>[6x]GPAMASEVLQKTRKINKTLQTSGGSSVSFDLLAGALGDVLSSNVYVVSAKGKVLGLHLNDV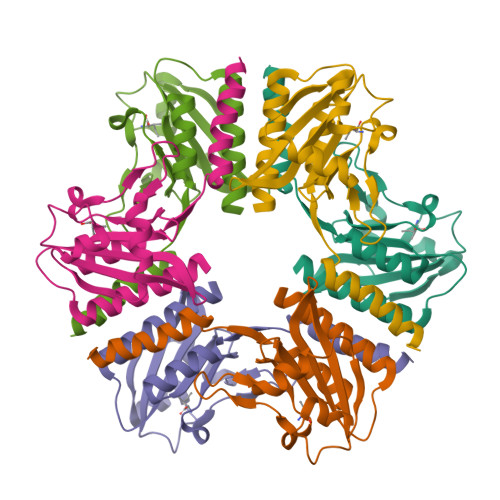QDSSVIEDEYTKQKKFSDEYTQNVLKIDETLENLNGEKILEIFPEEHGRLQKYTTVVPILGSGQRLGTLVLSRYSNSFNDDDLVIAEYSATVVGLEIL> SMSDVAIVKEGWLHKRGKYIKTWRPRYFLLKNDGTFIGYKERPQDVDQREAPLNNFSVAQCQLMKTERPRPNTFIIRCLQWTTVIERTFHVETPEEREEWTTAIQTVADGLK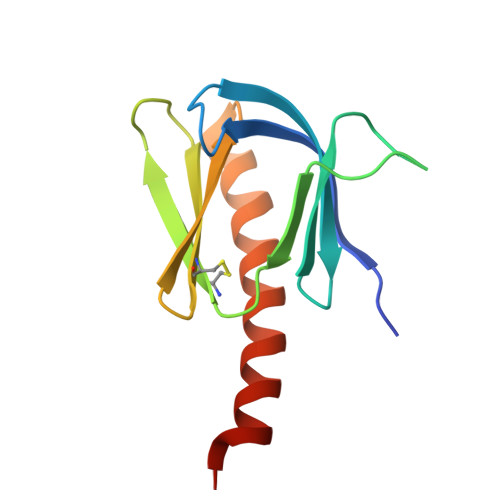KQEEEEMDFRSG>MAEESRGQRGSGYGLGLSTRTQVTGYQFLARRTAMALTRWRVRMEIEPGRRQTLAVVASVSAALVICLGALLWSFISPSGQLNESPIIADRDSGALYVRVGDRLYPALNLASARLITGRPDNPHLVRSSQIATMPRGPLVGIPGAPSSFSPKSPPASSWLVCDTVATSSSIGSLQGVTVTVIDGTPDLTGHRQILSGSDAVVLRYGGDAWVIREGRRSRIEPTNRAVLLPLGLTPEQVSQARPMSRALFDALPVGPELLVPEVPNAGGPATFPGAPGPIGTVIVTPQISGPQQYSLVLGDGVQTLPPLVAQILQNAGSAGNTKPLTVEPSTLAKMPVVNRLDLSAYPDNPLEVVDIREHPSTCWWWERTAGENRARVRVVSGPTIPVAATEMNKVVSLVKADTSGRQADQVYFGPDHANFVAVTGNNPGAQTSESLWWVTDAGARFGVEDSKEARDALGLTLTPSLAPWVALRLLPQGPTLSRADALVEHDTLPMDMTPAELVVPK[6x];>MQRFGTGSSRSWCGRAGTATIAAVLLASGALTGLPPAYAISPPTIDPGALPPDGPPGPLAPMKQNAYCTEVGVLPGTDFQLQPKYMEMLNLNEAWQFGRGDGVKVAVIDTGVTPHPRLPRLIPGGDYVMAGGDGLSDCDAHGTLVASMIAAVPANGAVPLPSVPRRPVTIPTTETPPPPQTVTLSPVPPQTVTVIPAPPPEEGVPPGAPVPGPEPPPAPGPQPPAVDRGGGTVTVPSYSGGRKIAPIDNPRNPHPSAPSPALGPPPDAFSGIAPGVEIISIRQSSQAFGLKDPYTGDEDPQTAQKIDNVETMARAIVHAANMGASVINISDVMCMSARNVIDQRALGAAVHYAAVDKDAVIVAAAGDGSKKDCKQNPIFDPLQPDDPRAWNAVTTVVTPSWFHDYVLTVGAVDANGQPLSKMSIAGPWVSISAPGTDVVGLSPRDDGLINAIDGPDNSLLVPAGTSFSAAIVSGVAALVRAKFPELSAYQIINRLIHTARPPARGVDNQVGYGVVDPVAALTWDVPKGPAEPPKQLSAPLVVPQPPAPRDMVPIWVAAGGLAGALLIGGAVFGTATLMRRSRKQQ[3x]

Specialized protein transport systems—known as type VII secretion systems (T7SSs)—are central to the virulence of this pathogen, and are also crucial for nutrient and metabolite transport across the mycobacterial cell envelope. Mycobacterium tuberculosis encodes five homologous, but functionally distinct, T7SSs that are designated ESX-1 to ESX-5. These systems translocate a number of effector proteins across the unique and impermeable diderm cell envelope. Here we reconstituted the ESX-5 T7SS of M. tuberculosis H37Rv in M. smegmatis to obtain a structural view of the entire T7SS membrane complex from this human pathogen.

The periplasmic assembly of the ESX-5 membrane complex of M. tuberculosis is formed by three EccB5 dimers and three MycP5 proteases. The EccB5 dimers assemble in a triangle, which forms a central cavity. Within an EccB5 dimer, two slightly different conformations (that is, inner and outer) can be distinguished between monomers, depending on their position. EccB5 dimerization is mediated mainly through the R1 and R4 repeat domains and is further stabilized by the EccB5 C termini, which wrap around their interacting EccB5 partner to form intermolecular hydrophobic contacts with its R1 domain. To form the triangle-shaped assembly, the inner EccB5 engages the outer EccB5 of the adjacent dimer by packing its R3 domain against the α-helices α5 and α8 of domains R2 and R3, respectively, which results in an asymmetric EccB5–tip arrangement. Our periplasmic M. tuberculosis ESX-5 map shows three MycP5 proteases that form a dome-like structure, which cap the periplasmic central cavity. Interactions between EccB5 and MycP5 are mediated mainly by the MycP5 protease domain and a composite interface that is generated by the R4 domain and loop 6 (residues Thr424 to Ser435) of the inner EccB5. The MycP5–EccB5 interface covers a surface area of about 1,230 Å2, which leads to the burial of three conserved tryptophan residues (Trp437 and Trp469 of EccB5, and Trp523 of MycP5). MycP5–MycP5 interactions are mediated mainly through loop 1 and the N-terminal extension (which run across the top of the MycP5 protomers), and loop 3, which contacts the neighbouring protease domain from the side. The active sites of the MycP5 proteases face towards the central lumen of the cavity, which implies that potential substrates of this protease are translocated through—and processed within—this periplasmic chamber.> GSFTYTFVVRDENSTVYAEVAKILLASGQWKRLKRDNPKFNLMLGERNRLPFGRLGHEPGLVQLVNYYRGADKLCRKASLVKLIKTSPELTETCTWFPESYVIYPTNEKTPAMRARNGLPDLANAPRTDEREEFRSSFNKKKENEEGNVWIAKSSSGAKGEGILISSDATELLDFIDNQGQVHVIQKYLESPLLLEPGHRK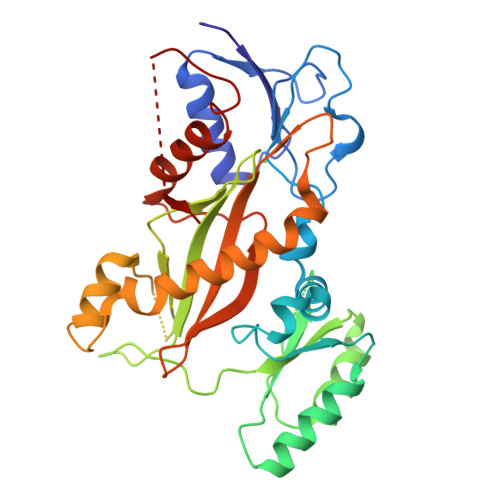FDIRSWVLVDNQYNIYLYREGVLRTSSEPYSDTNFQDMTSHLTNHCIQKEHSKNYGRYEEGNEMFFEEFNQYLVTSLNINLENSILCQIKEIIRVCLSCLEPAISTKYLPYHSFQLFGFDFMVDKNLKVWLIEVNGAPACAQKLYAELCKGIVDLAISSVFPLNEENHKPTEDNVFIKL> MAAACRSVKGLVAVITGGASGLGLATAERLVGQGASAVLLDLPNSGGEAQAKK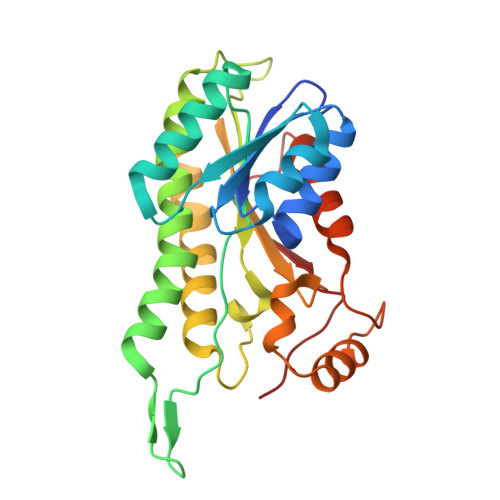LGNNCVFAPADVTSEKDVQTALALAKGKFGRVDVAVNCAGIAVASKTYNLKKGQTHTLEDFQRVLDVNLMGTFNVIRLVAGEMGQNEPDQGGQRGVIINTASVAAFEGQVGQAAYSASKGGIVGMTLPIARDLAPIGIRVMTIAPGLFGTPLLTSLPEKVCNFLASQVPFPSRLGDPAEYAHLVQAIIENPFLNGEVIRLDGAIRMQP> 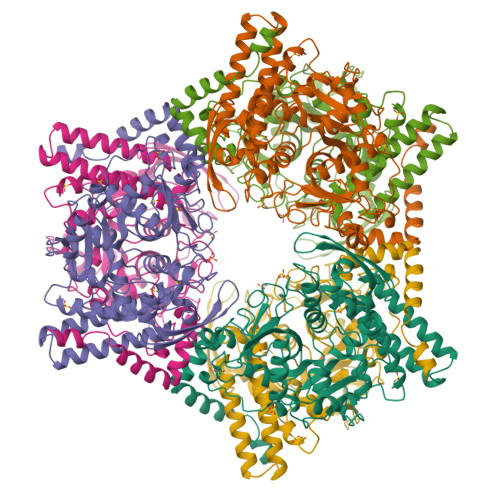MHHHHHHASENLAFQGAMASSIDISKINSWNKEFQSDLTHQLATTVLKNYNADDALLNKTRLQKQDNRVFNTVVSTDSTPVTNQKSSGRAWLFAATNQLRLNVLSELNLKEFELSQAYLFFYDKLEKANYFLDQIVSSADQDIDSRLVQYLLAAPTEDGGQYSMFLNLVKKYGLIPKDLYGDLPYSTTASRKWNSLLTTKLREFAETLRTALKERSADDSIIVTLREQMQREIFRLMSLFMDIPPVQPNEQFTWEYVDKDKKIHTIKSTPLEFASKYAKLDPSTPVSLINDPRHPYGKLIKIDRLGNVLGGDAVIYLNVDNETLSKLVVKRLQNNKAVFFGSHTPKFMDKKTGVMDIELWNYPAIGYNLPQQKASRIRYHESLMTHAMLITGCHVDETSKLPLRYRVENSWGKDSGKDGLYVMTQKYFEEYCFQIVVDINELPKELASKFTSGKEEPIVLPIWDPMGALAK>[8x]MTRLFMLVCLGIVCQGTTGNILRGESLNKSLPILHEWKFFDYDFGSDERRQDAILSGEYDYKNNYPSDIDQWHDKIFVTMLRYNGVPSSLNVISKKVGDGGPLLQPYPDWSFAKYDDCSGIVSASKLAIDKCDRLWVLDSGLVNNTQPMCSPKLLTFDLTTSQLLKQVEIPHDVAVNATTGKGRLSSLAVQSLDCNTNSDTMVYIADEKGEGLIVYHNSDDSFHRLTSNTFDYDPKFTKMTIDGESYTAQDGISGMALSPMTNNLYYSPVASTSLYYVNTEQFRTSDYQQNDIHYEGVQNILDTQSSAKVVSKSGVLFFGLVGDSALGCWNEHRTLERHNIRTVAQSDETLQMIASMKIKEALPHVPIFDRYINREYILVLSNKMQKMVNNDFNFDDVNFRIMNANVNELILNTRCENPDNDRTPFKISIHL;>[8x]MSKIVAVVVLAAFCVAMLVSDVSAKTSISVKGESNVDVVSQINSLVSSIVSGANVSAVLLAQTLVNILQILIDANVFA

Royal jelly (RJ) is a gelatinous, protein-, carbohydrate-, and lipid-rich secretion produced by the mandibular glands of nurse honeybees (Apis mellifera). At pH values below 4.5, as found in native RJ upon acidification in the mandibular glands, MRJP1 assembles with the small (5 kDa) RJ protein apisimin into long, hetero-polymeric filaments that can reach lengths above 1 µm12. These filaments were recently shown to be responsible for the high viscosity of RJ, guaranteeing that RJ-embedded queen bee larvae remain stably attached to the ceiling of the vertically oriented queen bee cells. Here we present the structure of native RJ filaments using a combination of cryogenic electron microscopy (cryo-EM) approaches based on tomography and helical reconstruction methods.

The resulting map, calculated at 3.5 Å resolution, was used for rebuilding the structure starting from the previous crystal structure and including the peripheral MRJP1 protein loops responsible for filament-forming inter-subunit contacts. Overall, we did not observe major conformational changes of MRPJ1 and apisimin in the RJ filaments with respect to the crystal structure determined at neutral pH. The resulting low-resolution ab initio reconstruction showed the overall architecture of the purified RJ filaments consisting of an H-shaped unit oligomerizing into a symmetric helical assembly by stacking interactions. The RJ helical assembly retains the D2 point group symmetry of the tetramers since both of the 2-fold rotational symmetry axes are orthogonal to the longitudinal axis of the filaments. Although the intrinsic flexibility of the N-linked glycans limits the map resolution at those sites, we were able to model one NAG residue at Asn28, two NAG residues at Asn144, and two NAG residues plus a β-D-mannose (BMA) residue at Asn177. The densities are ~25 Å long and are located at the center of the oligomer within a highly hydrophobic environment formed by the apisimin alpha helix 2 and the outer 24-methylenecholesterol from each asymmetric unit of the tetrameric oligomer. Although building an atomic model for this region was not possible, the highly hydrophobic chemical environment and the shape and length of the observed densities are consistent with a fatty acid with aliphatic tails of 12–16 carbons, or possibly a mixture of those. One of the contacts is mediated by homodimerization of MRJP1 alpha helices 1 (α1, residues 47–56) from neighboring building blocks that mainly interact via hydrophobic interactions involving Gln51, Ile54, and Leu55 of helix 1 as well as Tyr61 in the following loop. The helical assembly is further stabilized by a homodimerization interface present on the opposite side of the MRJP1 protein, involving homodimerization of a short turn (residues 280–281) followed by a loop segment (residues 287–295) that includes His294 and Asp292.NS1 is secreted alongside dengue virus particles during an infection. It is a multifunctional protein which exists in different oligomeric forms intracellularly and extracellularly, and they play distinctly different roles. The intracellular NS1 (iNS1), exists as a membrane associated dimeric form and is a part of the viral replication complex. The extracellular secreted NS1 (sNS1), exists in higher oligomeric forms. sNS1 likely causes vascular leakage symptoms in DHF/DSS via two pathways—indirectly, by stimulating the innate immune response through activation of complement and Toll-like receptors, and directly, by binding to endothelial cells causing endothelial hyperpermeability. sNS1 when bound directly to endothelial cells causes barrier dysfunction of the cell monolayer as demonstrated in an in vitro trans-endothelial electrical resistance (TEER) assay. Here we show by cryoEM that the recombinant sNS1 exists in multiple oligomeric states: the tetrameric (stable and loose conformation) and hexameric structures.

The 3.5 Å resolution recombinant sNS1 stable tetramer cryoEM map shows clear separation between β-strands. The density of both N- (residues 1–13) and C-terminal ends (residues 341–352) is missing from the map. Indeed, the space (25 Å) between two dimers within the stable tetramers is not big enough to accommodate the two iNS1 β-rolls. We observed that the β-roll densities, instead of concentrating at the middle of the dimers as observed in iNS1, have an elongated shape that stretches across the two protomers within a dimer. Fitting of the density map shows that residues 18–27 form a 27 Å long β-strand which pairs with the same β-strand of the other protomer within the dimer to form a long anti-parallel β-sheet (hereafter, referred to as elongated β-sheet). As the resolution of this region is ~4.5 Å, we analyzed their interaction by using a distance cutoff of 8 Å between the Cα backbone. Using this criterion, we observed that this elongated β-sheet from one dimer likely interacts with the same β-sheet from the opposite dimer via electrostatic interactions or hydrogen bonds at both ends of each respective β-sheet (Fig. 2c (i)–(ii)). Hydrophobic analysis shows that these β-sheets have an overall highly hydrophobic surface that also plays an important role in stabilizing their interactions. The iNS1 β-roll domain contains three β-strands (residues 1–7, 12–16, and 18–22), whereas we were unable to observe any density for residues 1–13 in the sNS1 stable tetramer, probably due to disorder in this region, and residues 18–27 form a long, continuous β-strand. Analysis of the epitopes on all NS1 molecules in the unbound stable tetramer shows they are only partially exposed (37.5%), thus discouraging Fab binding. While the Fab is able to cause dissociation between dimers in the loose tetramer and hexamer, it is unable to do the same to the stable tetramer.

>[4x]KELKCGSGIFITDNVHTWTEQYKFQPESPSKLASAIQKAHEEGICGIRSVTRLENLMWKQITPELNHILTENEVKLTIMTGDIKGIMQAGKRSLRPQPTELKYSWKAWGKAKMLSTELHNHTFLIDGPETAECPNTNRAWNSLEVEDYGFGVFTTNIWLKLKERQDVFCDSKLMSAAIKDNRAVHADMGYWIESALNDTWKIEKASFIEVKSCHWPKSHTLWSNGVLESEMIIPKNFAGPVSQHNYRPGYHTQTAGPWHLGRLEMDFDFCEGTTVVVTEDCGNRGPSLRTTTASGKLITEWCCRSCTLPPLRYRGEDGCWYGMEIRPLK> MDTMRQRILVVDDDASLAEMLTIVLRGEGFDTAVIGDGTQALTAVRELRPDLVLLDLMLPGMNGIDVCRVLRADSGVPIVMLTAKTDTVDVVLGLESGADDYIMKPFKPKELVARVRARLRRNDDEPAEMLSIADVEIDVPAHKV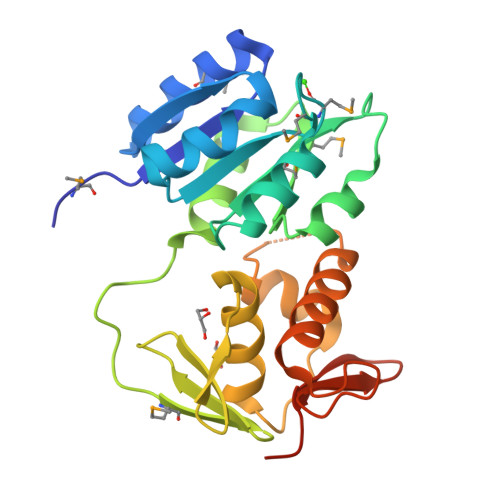TRNGEQISLTPLEFDLLVALARKPRQVFTRDVLLEQVWGYRHPADTRLVNVHVQRLRAKVEKDPENPTVVLTVRGVGYKAGPPTSGSHHHHHH>VTTSAPAQQIPFDFDNGNFIRDLITTHGGGGYPPADAMAPGDVSSYTWVTHLLQTSWFDALAPYHPTAVGVYSRIPRRPAEESATNRNKNIAGLYAMFQVVKAAFTERVPVLRQALGALGLDPDDESQDLSTAVGIGNTAGKAVAAARMGDGMNALGGKDRTHNGQPYEDYTGYRPVNTADELVDPSRWQPAVEPHRRRTDGGPGDKGIFTAQRFATPQLGLVAPQTYRDPARFKLAAPDHLDHNDAGAYRQAVDEVLAASAGLTDEQKVKAEFFEHTPLSVTLSPRAAAMAHDLDLDGWAQLFLVCSTARFDSLIAAWHHKRAYDTVRPFSAVRHVYGSKPVTAWGGPGKGTVESIPADEWTGYLPVGNHPEYPSGFTTLIAAQAQAARSFLGD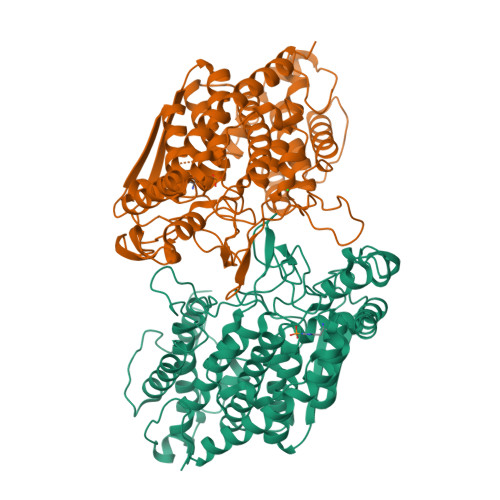DVLNWTHAFPAGSGQREPGAVPASDLELTWATWTDFENDCATSRVWAGAHFTKTAETSLAFGTQFGDLAHTFVQRHINGDVKD[2x]>[3x]MGKKMVVALGGNAILSNDASAHAQQQALVQTSAYLVHLIKQGHRLIVSHGNGPQVGNLLLQQQAADSEKNPAMPLDTCVAMTQGSIGYWLSNALNQELNKAGIKKQVATVLTQVVVDPADEAFKNPTKPIGPFLTEAEAK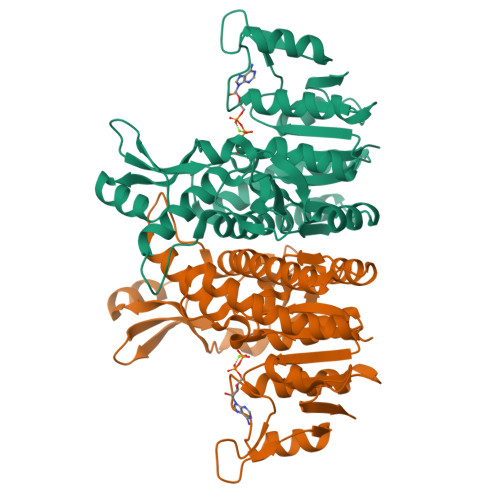EAMQAGAIFKEDAGRGWRKVVPSPKPIDIHEAETINTLIKNDIITISCGGGGIPVVGQELKGVEAVIDKDFASEKLAELVDADALVILTGVDYVCINYGKPDEKQLTNVTVAELEEYKQAGHFAPGSMLPKIEAAIQFVESQPNKQAIITSLENLGSMSGDEIVGTVVTK methyl 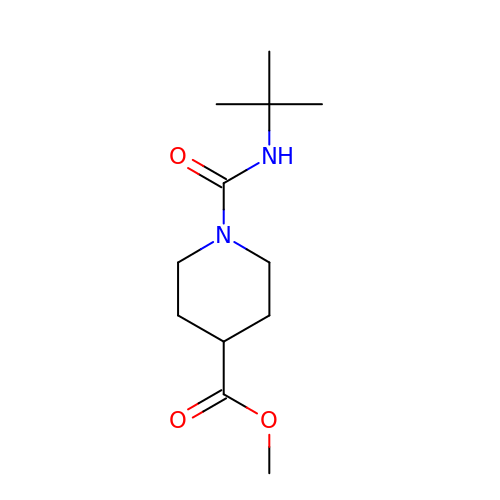1-(tert-butylcarbamoyl)piperidine-4-carboxylate | C12 H22 N2 O3 | YNDIZCMKDPECRX-UHFFFAOYSA-N>MHHHHHHQSWTSFVTPA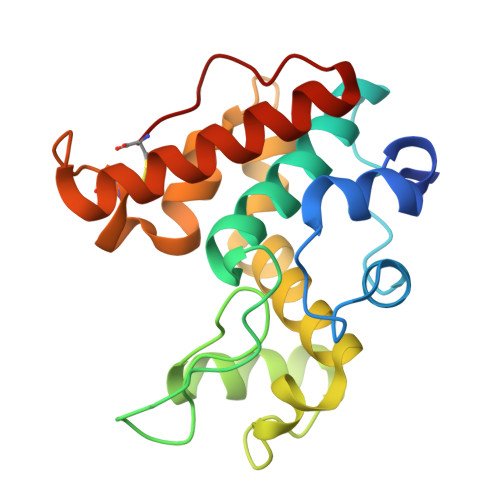VFEGWFPNRNPFYTYDGLVSASNGYPEFGTTGSLDDQKRELAAFLGNINQASGGLQFIQEQNPQSDQYYGRGPIQLSWNYNYGEAGADLGLDLLNNPDLVAQDSTVAWRTALWFWMKRDCHGAITASPPSFSGTIRIINGGLECNQPAGSIGNMQMENRVTYYTQFCQTLGVDPGTDLRC[3x]> KDLAMADLEQKVL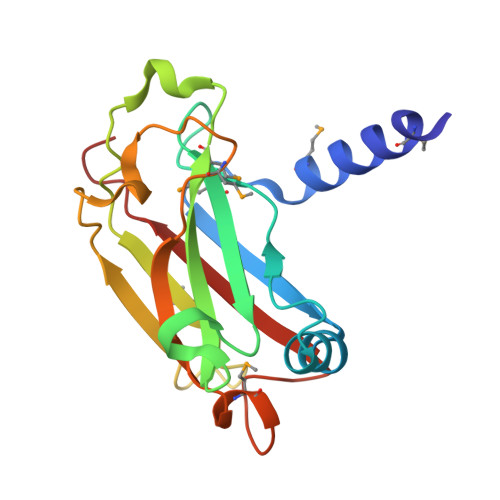EMEASTYDGVFIWKISDFPRKRQEAVAGRIPAIFSPAFYTSRYGYKMCLRIYLNGDGTGRGTHLSLFFVVMKGPNDALLRWPFNQKVTLMLLDQNNREHVIDAFRPDVTSSSFQRPVNDMNIASGCPLFCPVSKMEAKNSYVRDDAIFIKAIVDLTGL> MTDLKASSLRALKLMDLTTLNDDDTDEKVIALCHQAKTPVGNTAAICIYPRFIPIARETLKEQGTPEIRIATVTNFPHGNDDIDIALAETRAAIAWGADEVDVVFPYRALMAGNEQVGFDLVKACKEACAAANVLLKVIIETGELKDEALIRKASEISIKAGADFIKTSTGKVAVNATPESARIMMEVIRDMGVEKTVGFKPAGGVRTAEDAQKYLAIADELFGADWADARHYRFGASSLLASLLKALGHGDGKSASSYHHHHHH

2-Deoxy-d-ribose-5-phosphate aldolase (DERA) is used in organic synthesis for the enantioselective reaction between acetaldehyde and a broad range of other aldehydes as acceptor molecules. In 2001 the catalytic mechanism was resolved for DERA from Escherichia coli (DERAEC) by Heine et al.: the active K167 forms a Schiff base with the donor molecule, while K201 functions to reduce the pKa of K167 and, together with D102, participates in a proton-relay system critical for efficient catalysis. However, practical application of DERA in organic synthesis is limited by its poor stability towards high acetaldehyde concentrations. Hence, a monomeric variant of the enzyme (K58E-Y96W) was used that has virtually identical biochemical properties.

To determine the structure of these reaction product(s) and to identify the exact target site(s) within the protein, X-ray structures of DERA from E. coli before and after acetaldehyde incubation as well as after thermal treatment have been determined. Crystals were obtained for all three states under the same conditions, yielding datasets with resolutions ranging from 1.1 Å (native enzyme) to 1.5 Å (after heating). All three structures turned out to be very similar, with obvious alterations limited to the catalytic center. Interestingly, the native enzyme features electron density for a six-atom molecule with about 70% occupancy, which is attached to the active lysine residue. The covalent structure of this ligand is consistent with an aldol product formed by two acetaldehyde molecules (compound 2 in Fig. 4), which forms a hemiaminal (a hydrated Schiff base) with the lysine amino group. Given that this type of linkage is expected from the well-established catalytic mechanism of DERA, our findings may be rationalized by the presence of trace amounts of aldehydes in bacterial lysates or crystallization solutions. Importantly, this appears to be a reaction intermediate reflecting the intrinsic aldolase activity of the protein.Mitochondrial energy conversion requires an electron transport chain (ETC) that generates a proton motive force across the inner mitochondrial membrane to drive the essential adenosine triphosphate (ATP) formation by F1Fo-ATP synthase. The ETC consists of four multisubunit membrane complexes: complex I (CI; NADH:ubiquinone (UQ) oxidoreductase), complex II (CII; succinate:UQ oxidoreductase), complex III (CIII; cytochrome bc1) and complex IV (CIV; cytochrome c oxidase). We purified the intact respiratory supercomplex from mitochondria of the ciliate protist Tetrahymena thermophila and determined its structure by single-particle cryo-electron microscopy (cryo-EM). Here we show that a supercomplex containing all four respiratory chain components contributes to membrane curvature induction in ciliates.

CIV2 is the most divergent of the four ETC complexes. We modelled 105 lipids, four UQs and 53 protein chains per monomer, of which four are mitochondrially encoded. We found that two of those subunits, previously annotated as ciliate-specific Ymf67 and Ymf68 (also known as COX3) represent complementary protein fragments, with coding genes split in the mitochondrial genome by a tRNATrp gene insertion. Each fragment is extended by over 400 and 200 residues, respectively. Together, they form a functional COX3 (COX3a and COX3b), including the conserved seven transmembrane helix fold. In our structure, COX3a and COX3b extend throughout the CIV membrane region, and COX3b has evolved interactions with CI subunits on the matrix side, thereby mediating the supercomplex assembly. In particular, COX3b forms a contact with a peripheral amphipathic helix of NDUCA1, which is part of a zinc-free γ-carbonic anhydrase (γ-CA) heterotrimer. Another CI–CIV contact at the same site involves COXTT2 with a N-terminal globin-like domain that interacts with NDUFA3 and was not resolved in the individual CIV2 structure, suggesting that it becomes ordered to mediate supercomplex formation. Molecular dynamics simulations of CIV2 in a membrane suggest that it can also induce membrane bending in its immediate vicinity, similar to the supercomplex.

>MWVDFIDQTKSLKVSVNNYFYYLDRIKKLFTYLNDLRKHILKKYVYTINHKRIAINYLYFSMVTGLSGAALATMIRLELAHPGSPFFKGDSLRYLQVVTAHGLIMVFFVVVPILFGGFANFLIPYHVGSKDVAYPRLNSIGFWIQPCGYILLAKIGFLRPQFWRYYDKTSFSFPFLEKMKYNQYKEYKNDYLFYLDFLKKEITDDHSFFWKARKVIKLPQYSVFSFVPLKLMMWKTMINYPESFWYAASRVVQSRRKKVFVTKCSARTLTTAGWTFITPFSSNIKYTAVGSQDILILSVVFAGISTTISFTNLLITRRTLAMPGLRHRRVLMPFVTISIFLTLRMLATITPVLGAAVIMMAFDRHWQTTFFEYAYGGDPILSQHLFWFFGHPEVYVLIIPTFGFINMIVPHNNTRRVASKHHMIWAIYVMAYMGYLVWGHHMYLVGLDHRSRTMYSTITIMISMPATIKVVNWTLSLVNGALKIDLPFLFSMSFLLLFLVAGFTGMWLSHVSLNVSMHDTFYVVAHFHIMLSGAAMTGIFSGIYYYFNALFGVKYSRMFGYMHLIYYSGGQWVAFVPLFYLGFSGMPRRIHDYPVVFMGWHSMSTTGHFITLVGIIFFFLMMFDSHIERRASTSTTLGLPRWYKRISYYIFKIRYLQHTKSKMNGIPGSTVRLMLINRHFVEYEVYEK[2x];>MWGNLWTEASYQLNFNIGFSSLRSDVLIHLAQWQYWWWFWFALIWSFYYFIILKVARFRVLKMRPKISTSYRPHGKWGDFLACIIPLIWCINILTNSNLILRLIEWQNESSLFTVRVRARQWYWIYKFELKNFTDILSTPKNIGNNRWQINTFGELQTADDYLHVLQLRSQNKWVKNYWNRSLQETGKTNKAHVISPQEQLRLSLINQYKSLNLSSSIKHNAPFINRDLYVFDDLFSYNLGDITTKKSLFNDKNSFLTSYSYLNNNSWNNNEFDLIDNLPFTTLFDNNDLFNNYKSFFQDSIFNSPKKQLSSDSKQLFKHIIYRSIKNNIIQDYTKLVKHEDFDEYSRWIKRSPGEVLPLRIIKYPLGLETIHNNIFENTNNEGNVELFRLRFNSNSSKMQHKLVQDTIYLTLKQKRYNRKKVVAPQIKYYKDDNGNKTDLVKYTGKPYLSNDKLLKQSIYDQTTQYKLIKKNKKRGELIPVTLARRILRTKKTLVLPAHVNITLITNSYDIVHSWFIPGLGIKLDCVPGRSTHHTFFIDNVGFYYGQCAEICGRYHHHMPIRVCALPFEHFLLWWNTFGLPKMLNTVSRKRFETHYELRKYSW[2x];>[2x]MLICNFLMYSNFSRIYWFDFNGTVNENLPLNYNVLKICRNEINKLEKLNENNLGTQKNPIKLNLSFEDKHYNTNNLVLDLNSYETFNSKNFISSIFDKTFESLNTVLMAPIYSFLEFKLKLSSTKINTNHYYVINGKLYITYNDSFKLFTTINDYFNDLNELSNTKLFFLYRSFNIYNIKLNSLVDFVFLKLILFIHLLYLKSTNYNRFDYRLKQTDWGFYINNNSNYIQNIFSGLKYIWRGLRFWIIGLLLGLSSIYYLMYVRLLPFNKIIFAWILVAMFLYWLLSGFVFFVKKYQYSKFTAAIQRFWKRTYIIFWVIEAGTFSVFFYLTLNASSEPVYMYDQIKIYKTHLFSWRWFLIKLLPSVSIILLGYYLQLTLKWNLFNKQNTIVLLITLLLLYILWLEFYQFYHILSFYGNINWAFDYDEYIWTLELDTRRTRLANNYIAICLFAKFWHFVFIFLFWVFFVLRINELGRIRYPLLVANVQNFIIIYIMSWAYMYPWLKFIFRKYLDVPYYWFYLNGRELGIRVFFTDLKLFFYGITNRLFDFNPSSIKFEKYPFYYWINSSQLTEFNQYRKFVIRDSIIYSLNNYII;>[2x]MKKQKRTQGKQNTKQIKQEKLSSKRKANNQKEGKKKVKQEDYKEIKQKGKRMLSKIVKASFSSKGFNLANAVNTVKSTLNAPIKHIKRNIEPTGSNYSRMTNTTEEAFDEVSHEWQALVTSNPFDLNVFNYLENTQTSNFGTVDNPLVVFTSETPFRYVGCTGQMNEDDYEGHELLFFLLREGSLQRCMGCGQVFKLVRLRNEYSPEMDYYLSNFHPYEMQEMGESDTTVLMSPYKYASHYEYTQFETPSNMVYSMVNPDEHDRLLVDPAYRMERTKALEEKYKVYTSSLREVEKQFEERYGRAGQINISKVTYSTLIDVEKAVLKMDRLFRKVAKFENRAFIDRANHSRREKRMLERAQQRWDSNYSFFTGSLTEEEQKYRDYYETELEAYPEDEGIEQQLDQQEVLLSGRYDPKLYDFQEGYTKNPEDDQTSLIEKKAFKFRYRLANETSETFQRRNNRMVERQIKRFQQPQYKHAFEQLQKNIAISSNSGNALHSEYGYLELLSNESVQLYKDYYESDAEEDFKVFENLSSKEKLVMIANFENNLLPKYDRSEVHLIPKRQWEPAFGVWENFLYDITEYASFIAPRGKEIAADYQIQSAIPLTKEELIEAGLYKETIEKKVEPKLEAKKQTKSE;>[2x]MIWKYLQRTNRGNIIQAGLQHRKFENLPFKQNFDNLTKAYDLRMWYISNSPHEAKNLEYVNELEALHNELNYQNSRQFLFRTVSFLLGWALFYQFYELPKTYDWQDTQEPKHQVPAYGDLEEGGDEGGDD;>[2x]MSSAVEKKDLPADYGKMPAGYNFLTRGKDWREYDKDFILRTDAVWEKFQLEHFFRNYMKCFFFDHGLKKYQMFEPEDMYTVVFEGWALDDLITFPGFTPTGRTNSYQIGLSPRQRTVVPTQTFYQMQDYYMLCGLRFERWFRCDLVYHDQRHTKFDQVKNQKNYKTYPCYREYYEAQYACQDDMFDFLMELAYARRAADNFESDFASHELTTLPTFYDTPKAAERKTYTY;>MGSVWFRNRYWWYRSLYDDYVAREAKLAFGIAAFIWLPHYYWGIHLNRAFEVNFSHRNYAHEWGPRRNRLAHSLEFEQFDMILENWQDLEDEYAQRGDGMLKK[2x];>[2x]MNRFFKVSSKYQYYKYLEQYDAAFLRKYQSETHWYLGRRGAWKNLVIKYAGDHISLEEEHNVKYKTHLSFVYLSYRLAWVLFAYVLIYNHFLLGDIGKTFNVGEWDHRLKPSAERDYPTRYESLYILDRTQKW;>[2x]MISKYRYLHCARKLVKQSVQAFGGGHHHHEYDWRDDPKVNKDIEEDIRDRGWHPETYDFPYTKKHDDWVFDVTMPSQNYQTDLTVNIHPENKKMHVMKQVMRQSYWDAEHDMAHEYDYESEDLDFQCESFKSQHFRKKGPISQYLILGLLPILYFGTEFFYNHYPDEDYWRVAHPPPLDYPDTDDTDDTETFKDYKSFTGRRMVDTGIVDPLWYDIREGKKVYYDWAGVNQPMEDI;>MSLSLFGVKNNWHKNGIWWFSKILNKTVGEERYDALRVQRRIWSMRFYYARQQCLYELFVDHPDLAQWTGTYPKVDSSHGFPFYSTYEMYRDFQENTLNSDGSFAQWITLVCGIYVIHVIYNYMIPYYWVSTPLKNDEFTRLRMKDYIASTVLEEVYGISYAEWGWLPHDFAYNRMRGLAGYMHPDDPRAMCTSTFHRKHKYIEHEVEKVGDYHHMTYPK[2x];>[2x]MNKSQDEVKEDYFSIKKKKYNSLDCVLSPIVTRKKQESINSFQAGLQEDQNSTAVPESPFIRNCSETLNRSQHKILDHYFEYDYSLKKKIEKIKISLQNKTGTDSSQSLVQKRLDDLRKKTLIYKQFNIQKNNNNINNTGQFFIEKDKQNNLNLSQPHQIIKSKQGHKRSFTNTLYCSSNDKKIFNISSQKQNIKTVKQSNNSSMYEEQIKNDQNKKQNFNKQAKSERKQAEFCDLFYESMQKDAERQFKSNSDKSKSITQILENNCENAIVLLNHLIQILTDSIPISKNSILLDEKLSQCVNLSNNSKISQLMLVIQKLQGKISYYYNDFLKCIRMMKICKNFCQLFGTLKFKISCYKYIGLGFQRLNKPKVALVYFVKMLRQSWFLKQEDQEINSYDFIGMSYFYLGSIDKAYQYHQMMIDGIKADEEVKKISNIMLKNRKYSNYPTLQNIRIIQETSDGQPLQKTIRKSKIINPQFQLTQQEWGENISSSEDEFELPQMQIAVKNAEEQTFQKKFLSTPWNDRFIQAQIHKLEIAQELNYNKFPIGLVFKNQSVLNFPNSSNQPQLVVGPYANKIYNQELSSTYSSRQRISHQTPNREFFNYHSQLQQVKEQTQLNQMKQQYNQIVDSIELANHLIVLKNLKKVKDLFQNLIPYLNEKYYNIKQQNTKSLKQQQNSFDAQNSNQSFLGLQNYSIQINGILNINNQTDEYVNNQSDRSYQQQSDKLKLLIKSKSRNHSKEINMTQNYFKSPSNESKQIKNLRVIVDNSNKKKAQQKLNQEFSMNFCESPKYDNSILSLFINKLSQESALRLEIRQIGSASRYQRKKQQKGKQRKEKYQKKQEENKLNIKQYKKERYNMALFFMANTAISVPSVLDTSPCMKQMLAYEDCVLDANVPQQEVIHPQWPTIWPRLLTDGKLLEFDKVPFHPENIYNYTYMRPLTKKNKQYLYECEEERFVFKACLRKVISLKKTDKHTSWDTAEVANLQLT;>MYLFMHLCMCFCMISSSQKKEKLNKGKNKQIKLNKKKEKQNKKIEIIKKEKERRSNPQMISKTQAFARLFQLSSKSFSTVKGGNLYTWGQYASGTGFETASAVPRKVDYFSGNVSKVAMGPYHTAVITNDGSLYTFGWGQNGALGNGAKEFQLSPSGNLYTWGQYASGTGFETASAVPRKVDYFSGNVSKVAMGPYHTAVITNDGSLYTFGWGQNGALGNGAKEFQLSPSPVSFFNDKKLKVKDVVVGESYTIAVTENGEVYSWGYGGEPSSKINLDFFRNAILPQRCGALGSGDNKNRLTPQQIANLKADGYKNISGGDNFATLVNQSGEVINWGTGLFGSLGNGSDYPLFTPEVNAYFKHLKEHEGLTVQSIKSAGHFSAALLSNGKLYTFGVNTQGQLGIRENLGHNTDQNARLPTPVVDRHFVGQKVVDFEVGENTLVFLTDKNEVFFSGLELAYQPIRWEIPTDKKIVKLAASKDTFAAVTETGKIYQFNEFVGVSTNEVGNDYNVADSKAFEGKVVDLGGSYGIRFAIVN[2x];>[2x]MLSKVTRRFLNYNQIYCFASQHGAEHHKLTASDEAYLNEVRQRYVTPDMEKWAYLDYKKHPSTTLSHYDHKSKDYVESERDDYNADVATNSHNKLIDDFKRNLQMQRKVHDILQKMDRPYLRGVPGVTKNISAGLQDYSAPVSKKSQSDPNDFYRDAYRNENRWIDQSVFTPKTSKMTHYDVEWPKELASRPVTKKFHHDKGYKYDVTTPYDQRYNYVADRLGHPEILGNPFERLMRLEGDIYHPNYLDQPFVKVPNANPNASLNFEEGEVLYENTRLLEWAKFWNYSVVVGYLWCAYFVPYNIFFKTHMPLEHAYDNLFFPYFQHTHFLWDNNALHIPTVGGVAIYATYIALSYINNIWKDYVVRAQFSKDKELLFVTRVSPFGTTEEEVYEVAHLEHLPPSVRSGVKDLSAQDADGLVDVTCMSSQRSLVFYKGDQYWNPKVYNDFINQTSNLWTRNYTGYNRLEVQNSVEQVKIGFSHSSQPKLEKK;>MTALFLHILWSISYIIINILYIFLSLLLSNNNEKIKQYNSNYFIKILLVLFYNKNLSFYKNLLSEDEISKIEFERLKNYPTLVLIHSNLNKLEKRNKIINSFINFKTKYRFYKFISTNFNLQTIIKNCNDKIIFSTLLYIVNLNYSFFYKTIKNTDLIVYLLANKFSILNDNIIVSKFNISKFNDYIKYINNTNSIDTYLENQIILGLNNNTNSNITKNINTKLLNSYSNLKNLVNITNNTFYLKKINDNYNTVINSEFLTYLKSNYKISFSASNIVKYLSDKSVNNSVILYLRKNKIFNKSRYSRNRQTYRTGAYWCLYVNIIAVVAFYFWFYKFTMNFGYLWWLLYSLILSFFFSRALKHRFYNPLNVMTEFKNGFMWFIIILINIFKPLLKLLENNYINLYNHLVIKYYQSFICNTLINKKKLEFNYILSSFKFIKELNNIIIISLNKLF[2x];>MFRRIISNGALLSTQTQRWQDLSKFACLRASLNKESEKAFQELAKKNNVSPQELVELSKIVSMNLDVLKQNINSEQFLLEKESTLKRYRQSSIGTRGHLQTVNEAVNTKYPTLAEGLGQVAGYKEAYQALREIFVHPSISVNNLRQGSYGQQFAVDFRTRADEYVKALLKDHSSNPQAVQTIQEIQHTLHQIIKNYEQNPASIYARILTVLQTRGVNTLPVSKTADQKAVATIQKTSTPSLTIDQLTVPVQERVQTQTVFDAELAFIKEANEMIQQNTGNLPWDGGKKKIFQGQANKYLETPYYLLAALSGLGLLYFLYSGDAKYKTLVLTPVVGIAAFVLLRRNQILNRVPTLTELFLHKDGKFVDAVVSVNGQLISKNDIPVSTLKLYRGDHTVKVNLNDFEDASAKKFLAQQSGQEGVINVHFSKLRNLAARNGQVLNLGDTEVVVPFENQANRIILKQIFKGVEVLPSS[2x];>MYEGRWKMVNQIKQDVQNDIELILRQMNERIHAMKKKKYNELKGKIKQKCIDLLIDYAKQKIGKKNKIKKEGNNIRHNKQKKLKNIQKKIFKIISTRMLQTTLSAFRPRGSNVTGKVALATLGALTGYGAFYHYNQYLNLSARWQQIQENIAKDQPFDVDGFDAKVYPWVRENNVNDWEYKLVKMRGYFKDQRFFVRRKRDGKEGFLVFAPFVTAVERVNHRLKQKDLLPVEYSVFVNLGWVPVENKKDVELGGEVCPPMDAPTDSTLFVNDTFTGFNPDPANPEDTEQVTLTEITGIVRRGEQQDILARRRNWNKEGIYNWVDLDYMGKIFRLFNLDAINTAYIERVVPSFEEGEEGLYPIPATKDTFERPLNTPERHSTFFNFYAATSALSFISMLLLRR[2x];>MISARAVHRFLRNPNLETGAAFRAGTRFDPFKNTLTVLKDPQNGRTLYLIGTTNSSTLLANRTKDLVQKEKPDAVFVQTNKEWWNLAKNIQDVKCQQELNRYNDLLSQAYTLSLDNTIRNLVFKAKFYSWLFVINWFKAFPDDFHPFIPGLEMKFAIEEANKQNIPVVLGGLEVDDVTLSALKVEPRLDPFSQLYYGYRALHNSFWRREHFDNYATLDVVGGEAYAESMDRFRTNWFVKYFEKLAPYQKKIIVDQKDLDLFYALYRDTPGKKIVAVVNQWHVPGIENHWKSATNTHEPLKAINPIGDMDINKYMESQLVNDTLRAFVSKVGKTEPATWKNYSTIYHKDNYEAERVRHVAFVDHKDPHMYHGLPQDYDDNIKPKHH[2x];>[2x]MRYLKIEKEKLVSCKKQEQEVQRIRRRKGNQKLNSIAKQQRVKRRDYQQNIKQNKEVKNPKKLIKQQIINKVKKRKKMFRGLTKFNKVFALNSFKNSLVAVPKANLNHVQNMLEENLKYDAQKYNDEVAVIQKTSRIYKPTYTIEFNREGEVLVYSADPIKNSVVYFKYPYVLYEAAIPLFIWAWIYNPLELSKNAVNSLLIYPNIAWIPRMWYWRSLQYKIQKMYLLRGGKVAKIETQSLAGDRFTSWVETYQFHPLTQDQKNFDNQDNAEFLEDEGQLKYELGVQLDNLQEMGTTSQDIVINFMKEGTVHHPELFEAIVKGYNIDTSDYVINTANNLRAREGNHNH;>[2x]MFFELEDIKRRHSLYWDIYNVQGWVRRPDSTLYNNVKRGVTAGVVASLVQENITALVENCKLLATKYEKPQNLRQAATFMKEVFKLENYRKAVWNRSQYALCIGTFDIGARLATFRWLNNGWQRVFAGFEFNFVRKIPTTMLAALFTAPFSVPFELARMAYYGDKTFPKELQRGYSSYLSALARIPFEEGPYFLFKNSFPLIIRNFFQTFTLFYTYDFLKDKASFAWRVGEQNEYACKMIIAGISTYLAAVFSYPWMVTREMVDFWPKVPGAPCTFNGNYRKAAVWIWYHEFSGNYFAGFFTKYFWKASPGMFLTLMLADKVGLFDQTTVDNFGGAGNNSWEDTFV;>[2x]MFLNRLVKETSKAKRLFSMAQNNFARAGPYNPNRYKDYYIPRTLPKNEEIVEFVQSQHSVPASPIRNQRHINPVRESGPLPSYDGTYTMEDIRAVFYNTTVGRDYCYCQMDPEEIMRRVPGITRKEAEFITKLGLSPQEQVDFAYIAYNIGLDIFYFTNQMFVARQVVTNSKGEKVEVLWNAQCYEDIAQLNVGFAPVLESVDYHWEIFLWADPPIKPNNDFDLNVPCTWFEYEQEWWMESCIQEDQFNLPEDERPYNTPRNPHCRKELWRSQDALQEEELMVNENWYPKNTQYNIYNQPDFIKPKSGSGAAADDIRI;>[2x]MANFVIPYLKPVADFWNSLCIDQHQDSLFQFKGQTGSLGTDWTSKYLRSEQDVYNHKYLQYHKRVHEAPELTDVISDNVYRLTLFAGVERVLSVRQAQAILKTQFAGATENISGAFQTVLNGGIFRRGYFRGALLNLLQFCGAPYQSLIWSRNSGITNQVIVSSIFEAFFYPLDTVKTLIYNDVQGKYKGAFHCASQVVQNAGWSRLYAGIFQKLIFNSALIFHLNQVWDGSSQQWASLALVAAAYPLLVLKTRFQVAGTPLALATSNEVLKVNRKTLYAGLVPYLIFNTLFAYEFAAWHSSTAQERVIGGLQNAMKQFSSPAAEQVWSS;>[2x]MNYSYKRYWEPSTAEVIGLSLSVNTISAALTYPIEFVKVRSQIRTEGVGIRSKNLYMGINPNKVFREIHATGNGLRGFYQGFESHLIGRLSYLFIRNLTYKIIYDRTKPVKAHNDLSHREKGVIAGFAGGLAAFLTSPADLVNTRTIAEGGKPKEWRWGYKGLMDGINKIAATEGGNAALFRGSYANVLRAVILNISLTGPFDYLNEKIWITFGDMTWNKYAALLWASFWGSVATLPFDNIRTRLYAQNADPTKNRLTYSGWADAAKKLIQHEGISGFYVGFYAFYIRTFLYAWTTVFITDKITSDWKRKAGLKEWQI;>MLQQVFGKSKGGEVTNSHLTPKVLNKAQEAEKLASQIQAQRFSNRLVAFSSQYPRAKLFFAGIGIGTLLYGANQSSKARENKVATETRKERMAKPTIQLTGADSQNPPFTEKNINDWLYKTVSITGRPIHGKGMMIPAKSYGLHGFEYLVPFVTKENEDGSVQEGLILNLGFIPREYAPIWARARVENVEEQTFTCVVTDGKHLSEQGGLFASNKPCENQWEYADLDQLAKHTGFVNQEQVRSCILEHVNTETPNDERDCRHIDICSDYKEDYPYKFTRSGVLQQPGQMYWDLNKSASYYSLLGLGCSVFSALLFLAK[2x];>[2x]MVYHLFERICNPDNFKLSGEAARVRTLIAAGFSKEEAEQVAWLQNHQVNGKILGLFTGGFALYCCNNYFHYFERYFPRLRYQPFTKFLAQAATVYFFFKIGDYYFTSRRYGSNDARMNGLMYSNTYYSTNKEALIQNFEPLNRKFTEEEVEQFLRNEGRSQEEKRNWIYNPHIHGSTEGEWKADIHEKFDSGKAPWEREHVKAKILETNKAKIDAGEEIQLKPFKTLNHLDKTGLLHRLHPFIWTNNWTLLG;>MSSFIQYEFLKIYQGNQKIKNYYKRKRLIFQQKKVLKKKQKEIQMSTNNLRLKPWFHWTDEERSHAIFSAYEKRILKSEDLPSFLRANRINNVSTWVFPLIALPLFNQSIFKLGFAQRILLTRPAIEWHCFKIATVAASWLAWLNFSPFYRKLENEKEYLLDTLESRIGINVLDLNDALPRWTTSQEYNRRTQQLYNQRNGFFAGLLYPQEESSRPLVDIASFPKNLHKEKLTK[2x];>MFGRLVLKQTRRTLFNPVLKNTFCIYQAYQNPLRHINTGHNPNNVYEDIVMLGDYPVQNRTHDKVISQTYVPAIANIAFTHLSKKYPQAGLKVDQLNTLKEKTWNDLGVNIEHEKQEILVELSEQIFVKESKLRWVHEQRQRLAHTTYVFSGLEFQNVKVGFFIDSYNFLLQELAHRSNLYQSKDIVGEKSFHEKHLEQQTAPYSGVKSLEEPVSQNKSFINSLMRAIHNH[2x];>[2x]MYVLFVCLIDSMNVEEGKQIKEMILPHNNRQLARQYFDSLPENDINRKYYEGLKYETPKTFFGRFLNQFNIDAKLDTLSKFYTYQKTIRATQAELQEDRKSYLTNSLLFTAVSWFSIYQFARKGAVLPVLREYGRYFGTHRLFRQYLHTLVLPLLYTEYALNQKYYTHMEHLWTVHVNRLNQKILEDPLYTFYPQELNVPKHNIIVPTIFRDTPQ;>[2x]MKKGTASEEELKKLYDPNTFYEHGDNPAFKQFMNIAVENLREGKLTDHRTYVVDTYKKWMYARNWDDFLQRDCKAITFPRAFALWIVGTLGMATASKWCRQILPVGSHGITKISQTQFFHQFGPLGTLGAVGFYGLTAYLYYKTTIFTVKKFYSHCILQEREWIFEQERQNPGYGEYFFKDVPLSAEEHFNDLARGEMAKKKFEKPNHEF;>MSALLKEILALTVKSEAALWKGAEQKVLSGLNNLAKTELVQITHHFGVNKQGSEALWSQLDKAAVGAFPELSVDETLQLIDGFGECPDSYTLSHDLNQRLLVSWEQLGKLNFQKLKETNPYFASDIVNQLDAAAAEFIKVRPAAESEAGGFLNSLGVSSSFNTTKNDIYVVQSASGKKLNNKEQREAYVLEKAQKYLKEDPQSKILDIIAQK[2x];>[2x]MFLGIFKDVIKLLNKKVVPVYFWFFLYCFLSTMDTNIFVSSCSFLKVEVFGKDENTTLVLLFYVFYSLFNFYLSRIKNKNNYLVRKHLYTTELLIELILFKYKLIILKFSSIKYILNFNVRKFILFNLFLINNYKAYKINTFFLYIYIYLNNLNIIWYPIFKAYSIFGYYKSTRLNFIDTKNENIKRIKY;>[2x]MKEKIFNELTRKMKRKEISAKIQREENKQILIRQRNNKKYIQSIQGIQQERKKGKLYLVEMATQNVEEMDTIQKMNYEATVNMGRQDLITREYTFYSDYEFIPIQEDRKQQMEDALNNLHKIIHPTVTQLKKKANVQEIQDRVFRKLQGWEGELNTCVFSAKNVRDSNFCADRFTNRINTEGVEFVKQILREY;>[2x]MSAILKRAAKYKRVSSILCEGEAHLRDPFTPPPVILKPPAPRKDKKPDDITDFPAQKLIPLPESIPYQEGKYRPASIPMVAGFFPYNCYLQQGKVYSWCSCGISQSGPWCDGLCNSVVTRCRPVVFNVSQSGYYKICNCKFSANAPFCNNTHRKMVRYHHQTHRGFYEIWGAALFVLGWVYMGFNYYT;>[2x]MAARDFEYNNQDVNQLNGAFISLVEDEKIGFWVGVGGFAYSQFIMRKFVKSTNIFASVTSLFAGAALANLYTHQSRASYARVAARANRNASLALNKLMEY;>MDNNYHFWGNGDRQDVSLSYEDYYSILDCLLDEKLSPQGLMKFKNLHEVSMYGVSYVPLYCFPVAYGISHMLTGKVRRGHSGYRNLFSLMSVVLPFTCWYAYTTPIPRRLYTEIICSNNADGAYVRNRIKQQKPGIWRKLSQQLYNKNFRFPELNQDLTATEFPLDYVAPHKF[2x];>[2x]MVFEFLFYNQQHKTRNGYFINHDNLMLASLEERKKLIFYFIANQVPEKLDPVDRVKFNEELSDNLSTKARLIGSLTGLIGLVGFPYISTRIYSRPVLNIGLSLLICPFLYYVGNQLTYSVWEPKFIANNNTVCELSKKYNFTVFDFAQAKKEAHLKALRTELVSDNLLYSPGI;>[2x]MNNTFKFLHQVISKLTLKAQVPNYGQYSHSLKRPINPKVVVFGNSSRAYELISSQFRNFNHVNGLELKGQEDNIQANKVAQSVLSINDGFQDGYYITDFPQNSKQAERLDLITDGVNLALYIKDPSDKVTVTRQQEAIDYYRKTGALVEFEVDPRGDLEEQVKQLSNQVLNGYKH;>MAIRNFVFKISNQIQNLAAKRSLAYLNQIDSQSVPSRATINMKDQVTQMQREIDNMANVIRAQIPDEDRAEFEILKKYYVTGQHDSLVDPQDVLLQLDRIQVLKNLKMIELNEEAYDPELVRLEKLKARVLLEEEGALLEYAHFISKRPYNKPYEKWGVSEEHVKQQILG[2x];>MGFETVVPAPPTRDDELRMIKATEEQFLQQPRYKLYMNEAHRIAKMNHGDRHNNIRAHFWSNFALGLLITGPIFIIPFGKAFRNLRSGVPYYFRPKYVFTQKNQYNQDRNWGAMKKQIPLWLGLSTAYAYWFTDFSINDDEWLEKGKVIYPHQTIKVL[2x];>MSCTTRRFIDEKEKLEYSRGYNQQELEASKLRKDFVKKYIVDFDTTLYKTQVERDWAYIAKREYRYEVQLKSIGYGGALANAVLLWRIYANKKMVFWPIPIVGALGYLYFQPVFFQKSNKRFFDMCNVGEEYYLGRERNKILRECNKILNVEDF[2x];>MGKDQLDFSHFDKAFENKYDIVAPEFGDLHQKRAEFIAKNQGTYRPVPLVPNNIKGLIPKTCRLPATRNWYRRTSSFERNGFFNIHTPVLNTKMIPWLLFIVLTWGWSSFQIGGYNYERFDDNGERRNTLYWKLSPVEFPQSKLWNRPS[2x];>MVFHYTNFVQETNAWWLRRVRPVYCTVLAYYGWWLYDRYYLFGKNATQDIRKDTTEVWEKRAALNKRNWGYNAHYKPELERSMKKVLYADPNYKFPIEWPERYMAETKTLEQVMDEEENWEYYK[2x];>[2x]MMQNLKKFMSKTIQVQPVSFNQIPKAFYNFPEYRTGGVQANPGITAKRIIKCIGERLRKYDPARWENVPITFKTHFRDENGYSDVATSIQIHDALEREFGIDIKDRLALVTDVETAFYIVMSHHDPL;>[2x]MEPFGTDERNWTHEEKDIITRFLKYDKHVNLKTAEMVYSAEVESAYFGKAGALAGGVISALFFNFPIVRNLPIIRRSVIGVLPFLYCYTWGKNTQEELRWLKTFAAYQRFVVYHGQHCKLWV;>[2x]MAQTAHQNRYQGGLCYAQCNELFSFWNPSIQQCWKGCDFGVGRVNDPEGRIEAQQMCKRWAAELYWTYKGELDTIKDLRVHADMYPTTPQNVYRACLAGVRRQKF;>[2x]MFRWLFLYWYNSTDTPSAIAKVNLWSYINLRLFKARLSSSIAYYILGLNNLELKKLKIFYKNTYFDYIYLKSIPCLFLIIFFTNLYLFL;>MSTRKIFDSEEQSFIRLVDKFYLGLSLTKLCAQSCNLLRNDISGSALTQKEKDCLSICYNNIEKTQSAFYAKVKTTMNLPAVEDDGEEGGDDE[2x];>[2x]MSSDPFKKVERDYHNERSVHKHFASYPLKFWWGLNKFETIQGIHSILGNAADLVVSTLSFIPGVQGRNNASYIENSIRVTRFRGFDDKTQ;>MEVKYRGPSDDKLECEFLENNLLSCLREKSVQDNVAKMTCRPEFLVWFFLECPTKAAVYHDPKGLRNIFIQDKIKQKGSDDGVLSKDD[2x];>[2x]MEDNYAADVQRQFNRTAFDSLYKICYNSLVQKNGSTIDFQKQIDCHQRLIQVFAKIAPIVVKVEQDAASSGGAAAGGEDEE;>MSDKRKIQHEGIIALINYSTLCAQKCDVLKGHDDKITDTEEQCLRVCAEKIRQTFEFTNDIYLKNPNLTKPN[2x];>MDPVLGDVIATRIYKACFKHVYGKNMKAYSEKDEAKFDQCLTSYVESYKSVTNHFITYLGQLPKKGLSLDGS[2x];>[2x]MEQNTTQVFSDLAYKVCFKVINDKNKPFVLHDEQRLANCLTRYVEAFNVTSEYFFRERAGETKVTEKQ;>MDTEVSNHNYTQAVAYLNRATSSCVKKCDSLNNNGSLSSKQESCLKTCAENHAIATKIHAEYIRKLAESKYL[2x]> QEDEDGD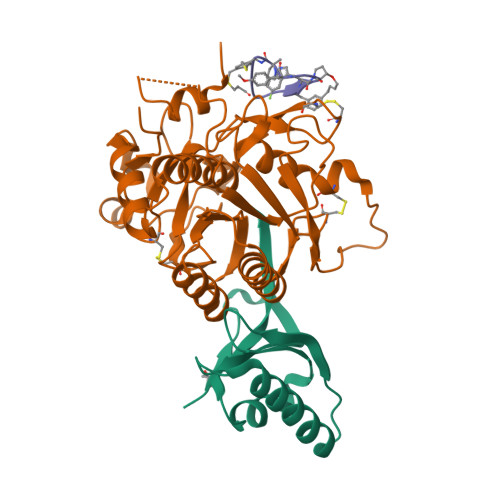YEELVLALRSEEDGLAEAPEHGTTATFHRCAKDPWRLPGTYVVVLKEETHLSQSERTARRLQAQAARRGYLTKILHVFHGLLPGFLVKMSGDLLELALKLPHVDYIEEDSSVFAQ;> SIPWNLERITPPRYRADEYQPPDGGSLVEVYLLDTSIQSDHREIEGRVMVTDFENVPEEDGTRFHRQASKCDSHGTHLAGVVSGRDAGVAKGASMRSLRVLNCQGKGTVSGTLIGLEFIRKSQLVQPVGPLVVLLPLAGGYSRVLNAACQRLARAGVVLVTAAGNFRDDACLYSPASAPEVITVGATNAQDQPVTLGTLGTNFGRCVDLFAPGEDIIGASSDCSTCFVSQSGTSQAAAHVAGIAAMMLSAEPELTLAELRQRLIHFSAKDVINEAWFPEDQRVLTPNLVAALPPSTHGAGNSHHHHHH>[8x]NSELDRLSKDDRNWVMQTKDYSATHFSRLTEINSHNVKNLKVAWTLSTGTLHGHEGAPLVVDGIMYIHTPFPNNVYAVDLNDTRKMLWQYKPKQNPAARAVACCDVVNRGLAYVPAGEHGPAKIFLNQLDGHIVALNAKTGEEIWKMENSDIAMGSTLTGAPFVVKDKVLVGSAGAELGVRGYVTAYNIKDGKQEWRAYATGPDEDLLLDKDFNKDNPHYGQFGLGLSTWEGDAWKIGGGTNWGWYAYD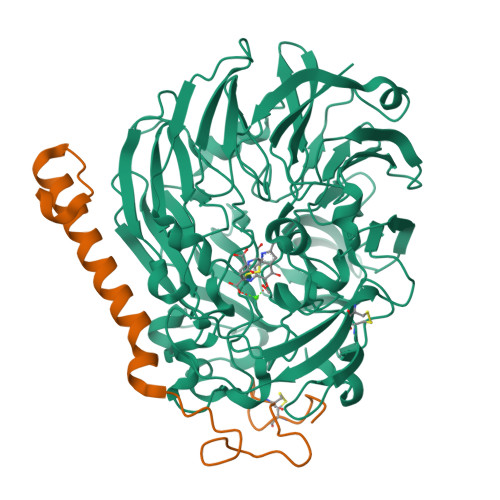PKLDMIYYGSGNPAPWNETMRPGDNKWTMTIWGRDADTGRAKFGYQKTPHDEWDYAGVNYMGLSEQEVDGKLTPLLTHPDRNGLVYTLNRETGALVNAFKIDDTVNWVKKVDLKTGLPIRDPEYSTRMDHNAKGICPSAMGYHNQGIESYDPDKKLFFMGVNHICMDWEPFMLPYRAGQFFVGATLNMYPGPKGMLGQVKAMNAVTGKMEWEVPEKFAVWGGTLATAGDLVFYGTLDGFIKARDTRTGELKWQFQLPSGVIGHPITYQHNGKQYIAIYSGVGGWPGVGLVFDLKDPTAGLGAVGAFRELAHYTQMGGSVFVFSL;>[8x]YDGTHCKAPGNCWEPKPGYPDKVAGSKYDPKHDPNELNKQAESIKAMEARNQKRVENYAKTGKFVYKVEDIK>GEEGNSSELPLSAEDAKKLTELAENVLQGWDVQAEKIDVIQGNQMALVWKVHTDSGAVCLKRIHRPEKKALFSIFAQDYLAKKGMNVPGILPNKK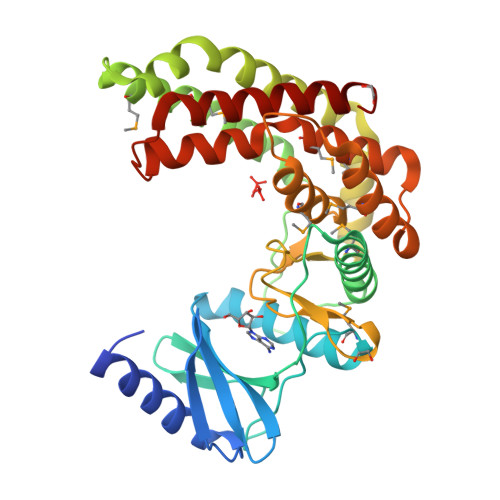GSLYSKHGSFLFVVYDWIEGRPFELTVKQDLEFIMKGLADFHTASVGYQPPNGVPIFTKLGRWPNHYTKRCKQMETWKLMAEAEKEDPFSQLYLQEIDGFIEDGLRIKDRLLQSTYVPWTEQLKKSPNLCHQDYGTGNTLLGENEQIWVIDLDTVSFDLPIRDLRKMIIPLLDTTGVWDDETFNVMLNAYESRAPLTEEQKQVMFIDMLFPYELYDVIREKYVRKSALPKEELESAFEYERIKANALRQLI[2x]>[2x]GAMSELSAIETAAAIAGGSMTALEACDAAIARIEQRDGPINAVVVRDFDRARDAAKAADAEIAAAVRKPLLGVPMTIKESFDIAGLPTSWGFAEHADHIATADSLVVSRLKAAGAVFLGKSNIPVGLADWQSVNPNYGRTNNPHDHSRSAGGSSGGAAAALAAGMVPLEYGSDIGGSIRVPAHFCGVWGLKTTFDAVSLEGHYFPRTDSAKADLSVVGPMARTPADLALALDITSKVPLPQSRIANLSGLRILLLTAHPETVADSATISAVERAAAACEASGATVATSSPDLPDLSALVADYTRMLLVVLARGLAPEGTEPVSLNAWYAMLDDQARMMRAFDRLFESFDAIFCPVLGTTAFAHSDEPDWAKRSLSIDGGIAPFAAQLGWISMATYGGMPALSMPLGADGNGLPINLQIITRNWSDHDAIRIGALVAEALDR

Here, the ligand‐free crystal structure of UMG‐SP2, a metagenome‐derived urethanase with depolymerization activities, at 2.59 Å resolution, as well as its (co‐)structures bound to a suicide hydrolase inhibitor and a short‐chain carbamate substrate at 2.16 and 2.40 Å resolutions, respectively, is reported. UMG‐SP2 belongs to the amidase signature protein superfamily (AS family), which is characterized by a highly conserved GGSS(S/G)GS motif and can be found in bacteria, archaea, and eukaryotes. SP2 shares the domain architecture of amidases, with an α/β‐fold containing 12 prominent α‐helices, 12 β‐strands, and five larger loops. Structural analysis and molecular dynamics simulations reveal that the flexible loop L3 consisting of residues 219–226 is crucial for regulating the hydrolytic activity of UMG‐SP2.

The crystal structures of wild‐type (WT) UMG‐SP2 (GenBank Accession No. OP972510) were solved in a substrate‐free state (SP2, also used as an interchangeable designation for WT UMG‐SP2 for simplification, 2.59 Å resolution) and a complex with the phenylmethylsulfonyl moiety of the suicide inhibitor PMSF covalently bound to the active site serine 190 (SP2PMS, 2.16 Å resolution). The structures of SP2S190A and SP2 were solved by MR based on the refined structure of SP2PMS omitting the covalently modified S190. Due to the hydrophobic nature of the entire active site cavity, two glycerol molecules from the cryoprotectant solution were found bound to the active site in the substrate‐free structure, one of which contacted the backbone of the oxyanion hole residues (left inset). In the ligand‐free structure, A141 is in the vicinity of a glycerol molecule. In SP2 and SP2PMS, K224 (part of L3 at the perimeter of the secondary active site cavity) interacts with several water molecules and H215 (as well as S222 in the SP2 structure). These interactions consolidate K224 pointing toward the substrate binding cavity and blocking the secondary active site sterically (right insets). The surface of SP2 is largely negatively charged, but positive charge overweighs the substrate‐free structure in the primary and secondary active site cavities, in contrast to the BBC‐bound SP2S190A. This charge difference is also the result of the aforementioned structural switch that distinguishes SP2 from the substrate‐bound complex structure of SP2S190A. Due to the steric blockage of the active site when empty or partially occupied by PMS, substrate accessibility (in particular for larger molecules) is limited, in contrast to the complex structures with one or two BBC molecules bound.> ELPQMTQQLNSDDMQEQLSATVKFRQILSREHRPPIDVVIQAGVVPRLVEFMRENQPEMLQLEAAWALTNIASGTSAQTKVVVDADAVPLFIQLLYTGSVEVKEQAIWALGNVAGDSTDYRDYVLQCNAMEPILGLFNSNKPSLIRTATWTLSNLCRGKKPQPDWSVVSQALPTLAKLIYSMDTETLVDACWAISYLSDGPQEAIQAVIDVRIPKRLVELLSHESTLVQTPALRAVGNIVTGNDLQTQVVINAGVLPALRLLLSSPKENIKKEACWTISNITAGNTEQIQAVIDANLIPPLVKLLEVAEYKTKKEACWAISNASSGGLQRPDIIRYLVSQGCIKPLCDLLEI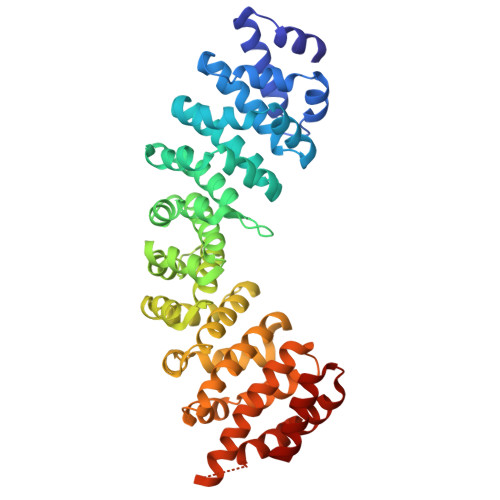ADNRIIEVTLDALENILKMGEADKEARGLNINENADFIEKAGGMEKIFNCQQNENDKIYEKAYKIIETYFG>MADDQGCIEEQGVEDSANEDSVDAKPDRSSFVPS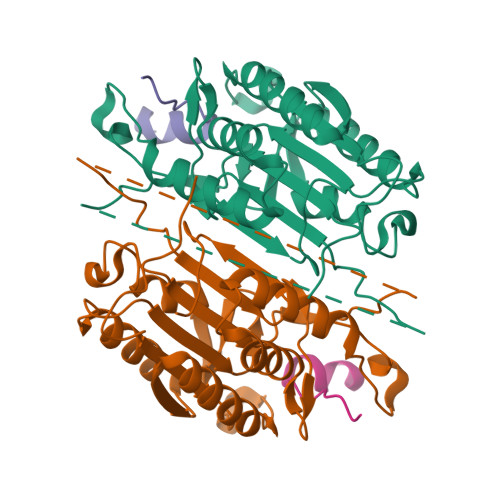LFSKKKKNVTMRSIKTTRDRVPTYQYNMNFEKLGKCIIINNKNFDKVTGMGVRNGTDKDAEALFKCFRSLGFDVIVYNDCSCAKMQDLLKKASEEDHTNAACFACILLSHGEENVIYGKDGVTPIKDLTAHFRGDRCKTLLEKPKLFFIQAARGTELDDGIQADSGPINDTDANPRYKIPVEADFLFAYSTVPGYYSWRSPGRGSWFVQALCSILEEHGKDLEIMQILTRVNDRVARHFESQSDDPHFHEKKQIPCVVSMLTKELYFSQ[2x];>[2x]RDHFALDRPSETHADYLLRTGQVVDISDTIYPRNPAMYCEEARLKSFQNWPDYAHLTPRELASAGLYYTGIGDQVQCFCCGGKLKNWEPCDRAWSEHRRHFPNCFFVLGRNLNIRSESD>GGAHKVRAGGPGLERAEAGVPAEFSIWTREAGAGGLAIAVEGPSKAEISFEDRKDGSCGVAYVVQEPGDYEVSVKFNEEHIPDSPFVVPVASPSGGASGSGASGSSGSWKVGFF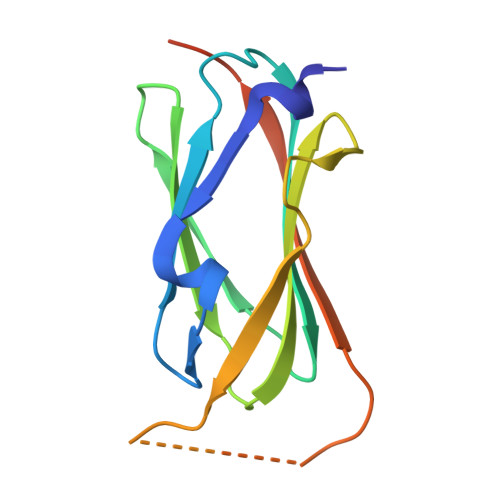KRNRPPLEEDDEEGEG[2x]>[2x]MPASAPPRRPRPPPPSLSLLLVLLGLGGRRLRAEPGDGAQTWARFSRPPAPEAAGLFQGTFPDGFLWAVGSAAYQTEGGWQQHGKGASIWDTFTHHPLAPPGDSRNASLPLGAPSPLQPATGDVASDSYNNVFRDTEALRELGVTHYRFSISWARVLPNGSAGVPNREGLRYYRRLLERLRELGVQPVVTLYHWDLPQRLQDAYGGWANRALADHFRDYAELCFRHFGGQVKYWITIDNPYVVAWHGYATGRLAPGIRGSPRLGYLVAHNLLLAHAKVWHLYNTSFRPTQGGQVSIALSSHWINPRRMTDHSIKECQKSLDFVLGWFAKPVFIDGDYPESMKNNLSSILPDFTESEKKFIKGT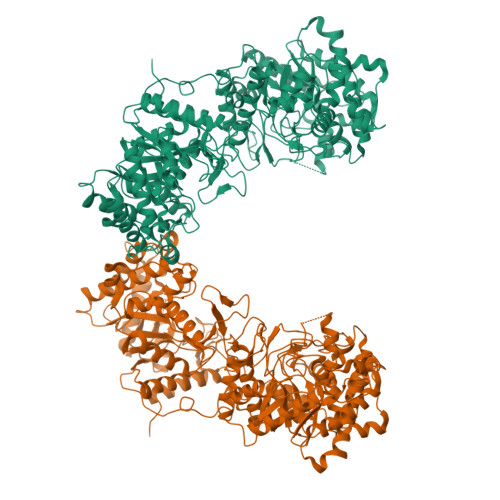ADFFALCFGPTLSFQLLDPHMKFRQLESPNLRQLLSWIDLEFNHPQIFIVENGWFVSGTTKRDDAKYMYYLKKFIMETLKAIKLDGVDVIGYTAWSLMDGFEWHRGYSIRRGLFYVDFLSQDKMLLPKSSALFYQKLIEKNGFPPLPENQPLEGTFPCDFAWGVVDNYIQVDTTLSQFTDLNVYLWDVHHSKRLIKVDGVVTKKRKSYCVDFAAIQPQIALLQEMHVTHFRFSLDWALILPLGNQSQVNHTILQYYRCMASELVRVNITPVVALWQPMAPNQGLPRLLARQGAWENPYTALAFAEYARLCFQELGHHVKLWITMNEPYTRNMTYSAGHNLLKAHALAWHVYNEKFRHAQNGKISIALQADWIEPACPFSQKDKEVAERVLEFDIGWLAEPIFGSGDYPWVMRDWLNQRNNFLLPYFTEDEKKLIQGTFDFLALSHYTTILVDSEKEDPIKYNDYLEVQEMTDITWLNSPSQVAVVPWGLRKVLNWLKFKYGDLPMYIISNGIDDGLHAEDDQLRVYYMQNYINEALKAHILDGINLCGYFAYSFNDRTAPRFGLYRYAADQFEPKASMKHYRKIIDSNGFPGPETLERFCPEEFTVCTECSFFHTRKSLLAFIAFLFFASIISLSLIFYYSKKGRRSYK Many protein families have numerous members listed in databases as allergens; however, some allergen database entries, herein called “orphan allergens”, are members of large families of which all other members are not allergens. Three orphan allergens [Cladosporium herbarum aldehyde dehydrogenase (ChALDH), Alternaria alternata ALDH (AaALDH), and C. herbarum mannitol dehydrogenase (ChMDH)] were recombinantly produced and purified for structure characterization and for clinical skin prick testing (SPT) in mold allergic participants. Diffraction quality crystals of ChALDH and ChMDH were obtained, and their X-ray crystal structures were determined by molecular replacement. Examination of the X-ray crystal structures of ChALDH and ChMDH and a homology structure model of AaALDH did not identify any discernable epitopes that distinguish these putative orphan allergens from their non-allergenic protein relatives.

ChMDH is also a member of a broadly represented superfamily of multimeric enzymes (i.e., short-chain dehydrogenases/reductases (SDR) superfamily) that catalyzes the oxidation and reduction of various alcohols in multiple organisms. The three-dimensional structure of ChMDH (the third orphan allergen selected for study) in complex with NADP+ was determined at 2.04 Å resolution. ChMDH is a tetrameric protein in the X-ray crystal structure and in size-exclusion chromatographic analysis. In both sequence and three-dimensional structure, the monomeric unit of ChMDH is defined by the Rossmann-fold observed in multiple nicotinamide-dependent enzymes, which is conserved across members of the SDR enzyme superfamily, that includes MDH from various species. Clear electron density for NADP+ in the ChMDH·NADP+ complex was observed and identified the active site in the enzyme. The residues of the nicotinamide cofactor binding site in ChMDH are highly conserved with other SDR family members. As expected, ChMDH showed the highest similarity with other members of the SDR enzyme family, which ranged in amino acid sequence identity from 26 to 45% with 1.1 to 1.7 Å r.m.s.d. for 237–264 Cα-atoms. Although the amino acid sequence of ChMDH shares low sequence identity (~ 30%) with the SDR family members from portobello mushroom, canola, and human, the pairwise structural comparisons between ChMDH and these enzymes underscores the evolutionary conservation of the protein fold in each. Comparison of the surface features of ChMDH and the representative SDRs from portobello mushroom, canola, and human reveals some variation in the electrostatic potentials of the proteins, especially in the oligomerization interfaces, but are similar in their surface hydrophobicity.

>[8x]GSHMPGQQATKHESLLDQLSLKGKVVVVTGASGPKGMGIEAARGCAEMGAAVAITYASRAQGAEENVKELEKTYGIKAKAYKCQVDSYESCEKLVKDVVADFGQIDAFIANAGATADSGILDGSVEAWNHVVQVDLNGTFHCAKAVGHHFKERGTGSLVITASMSGHIANFPQEQTSYNVAKAGCIHMARSLANEWRDFARVNSISPGYIDTGLSDFVPKETQQLWHSMIPMGRDGLAKELKGAYVYFASDASTYTTGADLLIDGGYTTR> MSPAKEQDRFLPIANVSRIMKRSLPANAKISKEAKETVQECVSEFISFVT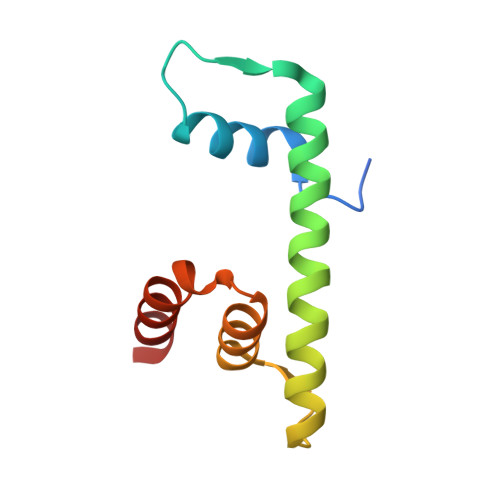GEASDKCQREKRKTINGDDLLWAMTTLGFEAYVGPLKSYLNRYRE>[2x]MRQVDAATHGGRAVIELREKILSGELPGGMRLFEVSTAELLDISRTPVREALSRLTEEGLLNRLPGGGFVVRRFGFADVVDAIEVRGVMEGTAARLAAERGVSKVALEEIDATVQQLDLCFGDRVDDVDFDGYAALNRIFHHQLAALCGSEMIRREVERASSLPFASPSAFLPDKANIGAFRRSLRGAQEQHKAIVAAIVAREGARAEAVAREHSRTARTNLEYMIREAPELIAQVPGLALISDHHHHHH

Here, we characterized Atu1419 as a transcriptional repressor of its own repression in addition to two other genes (atu1418 and atu1420). The structures revealed Atu1419 to be a member of the VanR group of the FadR C-terminal domain (FCD; Pfam PF07729) subfamily of the large GntR superfamily of transcriptional factors (>93 135 members in Pfam database). Like FadR, Atu1419 possesses a characteristic molecular architecture, composed of a conserved N-terminal DNA binding domain containing the wHTH motif and a C-terminal effector binding/oligomerization domain. We identified the short palindromic region composed of 10 base pairs and a degenerated palindrome bound to Atu1419 and the N5,N10-methylenetetrahydrofolate (MEF) as the effector molecule disrupting Atu1419-DNA interaction, allowing the expression of the second part of the HCA degradation pathway.

The structures of two palindromic DNA-Atu1419 complexes solved at 2.79 Å resolution (P6422 space group) and 2.05 Å resolution (C2221 space group) present a distinct neighboring crystal packing with an asymmetric unit containing a monomer bound to a single DNA strand and a dimer bound to the 10-mer palindromic DNA, respectively. Nonetheless, a tetramer, where dimers AB and CD bind each to a DNA palindrome, was reconstituted by crystal symmetries in line with the conservation of Atu1419 tetramer in solution upon DNA binding. The three monomers of the asymmetric units (one in P6422 and two in C2221) are similar with an average RMSD value of 1 Å for all Cα atoms making almost identical interactions with DNA, although the positions of the DNA binding domains within the dimers between the two crystal structures do not completely overlap. Each monomer recognizes a half-site DNA with helices α2 and α3 of the HTH motif making nine polar interactions with both strands in the major groove of the DNA. Helix α3 via Ser44, Thr46, Arg45 and Arg49 side chains is responsible for six hydrogen bonds with both strands, half with oxygens of phosphate groups 5′ of guanine (G3) at position 3 on one strand and of adenine (A5) at position 5 on the complementary strand. The other half is made by the guanidinium group of Arg45, which provides specific contacts with the N7 and O6 atoms of G3 on one strand and by OG1 of Thr46 with the N7 of A5 on the other strand. The remaining H-bonds come from helix α2 via the Arg31 side chain and the main chain amino group of Glu34, and an additional interaction is present with the main chain NH of His9 in helix α1. They consist of phosphate contacts with A1 and T2 on one DNA strand and T4 on the other. All Atu1419-DNA subunits contain a bound Zn2+ ion at the same position as that observed in both Atu1419–citrate complexes. In contrast to the protein-DNA complex in C2221 space group, which crystallized in MES buffer, the P6422 protein–DNA complex reveals a bound citrate in the effector binding pocket.Here we present a strategy for fusing small RNAs to a group II intron that yields high resolution structures of the appended RNA. Group II introns are self-splicing catalytic RNAs that have six distinct domains and typically range in size from 400 to 850 nucleotides. Our versatile scaffolding strategy enables efficient RNA structure determination for a broad range of small to moderate-sized RNAs, which were previously intractable for high-resolution cryo-EM studies.

We attached the aptamer domain of the thiamine pyrophosphate (TPP) riboswitch14 (86-nt) to our group II intron scaffold (O.i.-TPP). The TPP riboswitch was covalently attached to the solvent exposed domain III stem of the O.i. group IIC intron through a rigid helix. SHAPE-MaP31 confirmed that the secondary structure of the 493-nt linked group II intron and riboswitch structure maintained the expected fold for both RNA domains. Cryo-EM data collection and subsequent processing were performed for the scaffold attached to the riboswitch. Clear additional signal, corresponding to the attached riboswitch, was visible in all 2D class averages as compared to the 2D classes of the scaffold alone. Local refinement, focused on the scaffold, yielded a 3D reconstruction with a resolution of 2.4 Å for the core of the intron. A comparison of the resulting maps and models for the scaffold alone and with the TPP riboswitch embedded shows that the attachment process did not affect the overall fold of the scaffold. The locally refined map of the scaffold maintains high-resolution features after the TPP riboswitch is embedded. The viewing distribution plot shows that embedding the riboswitch did not create a preferred orientation for the overall fusion construct.

> GUUAUGUGUGCCCGGCAUGGGUGCAGUCUAUAGGGUGAGAGUCCCGAACUGUGAAGGCAGAAGUAACAGUUAGCCUAACGCAAGGGUGUCCGUGGCGACAUGGAAUCUGAAGGAAGCGGACGGCAAACCUUCGGUCUGAGGAACACGAACUUCAUAUGAGGCUAGGUAUCAAUGGAUGAGUUUGCAUAACAAAACAAAGUCCUUUCUGCCAAAGUUGGUACAGAGUAAAUGAAGCAGAUUGAUGAAGGGAAAGACUGCAUUCUUACCCGGGGAGGUCUGGAAACAGAAGUCAGCAGAAGUCAUAGUACCCUCAGUACUCGGGGUGCCCUUCUGCGUGAAGGCUGAGAAAUACCCGUAUCACCUGAUCUGGAUAAUGCCAGCGUAGGGAAGUGCUGAGGGGAAGGACGGAACAAGUAUGGCGUUCGCGCCUAAGCUUGAACCACCGUAUACCGAACGGUACGUACGGUGGUGUGAGAGGAGUUCGCUCUACUCUAU> MEYTTDIPAVFTDPSVMERYYYTLDRQQSNTDTSWLT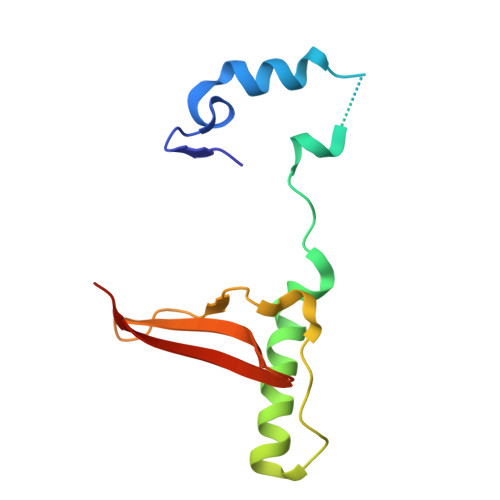PPQLPPQLENVILNKYYATQDQFNENNSGALPIPNHVVLNHLVTSSIKHNTLCVASIVRYKQKYVTQILYTPIESS(2E)-3-(3-bromo-4-hydroxyphenyl)prop-2-enoic acid | C9 H7 Br O3 | 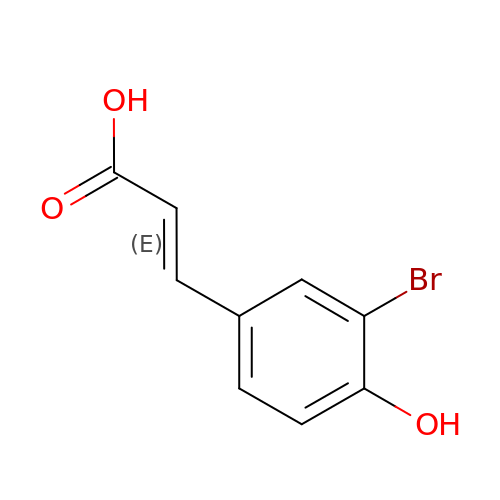HOZXBZABAJSGDX-DUXPYHPUSA-N Varicella-zoster virus (VZV) is a highly infectious, human host restricted alphaherpesvirus that causes varicella (chickenpox), establishes latency in sensory ganglion neurons and can reactivate to manifest as zoster (shingles). Herpesvirus virions have an outer lipid membrane studded with glycoproteins that enable fusion with cell membranes to initiate entry and establish infection. The most conserved herpesvirus protein, glycoprotein B (gB), is classified as a type III fusogen due to its structural similarities with vesicular stomatitis virus (VSV) G protein and baculovirus gp64. In contrast to these fusogens, gB requires additional virally encoded glycoproteins, gH and gL, which are implicated in membrane binding and priming of the gB trimer, to induce membrane fusion.

The VZV gB ectodomain was composed of five domains, DI to DV, with 13 helices and 31 β-strands, similar to herpesvirus orthologue structures in their postfusion conformations. Each protomer was stabilized by five disulfide bonds, conserved among alpha-, beta-, and gammaherpesviruses. C122/C584 stabilized the non-contiguous regions of DIV (N-terminal, aa115-136 and C-terminal, aa570-681) and C139/C540 bridged the distal end of the long central helix of DIII (α8) with the linker to DII.

>[2x]MSPCGYYSKWRNRDRPEYRRNLRFRRFFSSIHPNAAAGSGFNGPGVFITSVTGVWLCFLCIFSMFVTAVVSVSPSSFYESLQVEPTQSEDITRSAHLGDGDEIREAIHKSQDAETKPTFYVCPPPTGSTIVRLEPPRTCPDYHLGKNFTEGIAVVYKENIAAYKFKATVYYKDVIVSTAGAGSSGTQITNRYADRVPIPVSEITDTIDKFGKCSSKATYVRNNHKVEAFNEDKNPQDMPLIASKYNSVGSKAWHTTNDTYMVAGTPGTYRTGTSVNCIIEEVEARSIFPYDSFGLSTGDIIYMSPFFGLRDGAYREHSNYAMDRFHQFEGYRQRDLDTRALLEPAARNFLVTPHLTVGWNWKPKRTEVCSLVKWREVEDVVRDEYAHNFRFTMKTLSTTFISETNEFNLNQIHLSQCVKEEARAIINRIYTTRYNSSHVRTGDIQTYLARGGFVVVFQPLLSNSLARLYLQELVRENTNHSPQKHPTRNTGSGGSVPVELRANRTITTTSSVEFAMLQFTYDHIQEHVNEMLARISSSWCQLQNRERALWSGLFPINPSALASTILDQRVKARILGDVISVSNCPELGSDTRIILQNSMRVSGSTTRCYSRPLISIVSLNGSGTVEGQLGTDNELIMSRDLLEPCVANHKRYFLFGHHYVYYEDYRYVREIAVHDVGMISTYVDLNLTLLKDREFMPLQVYTRDELRDTGLLDYSEIQRRNQMHSLRFYDIDKVVQGSHHHHHH The method of serial femtosecond crystallography (SFX) has pushed the frontiers of protein crystallography at X-ray FELs through the use of smaller crystals than typically used with conventional sources and the use of the unique time resolution afforded by X-ray FELs131415. For SFX to contribute novel structural information, routine de novo phasing from X-ray FEL data is necessary. Extending the Se-SAD phasing ‘magic bullet' of structural biology to SFX experiments promises to provide a routine method for de novo phasing at X-rays FELs.

Here we show the successful use of single-wavelength anomalous diffraction to solve the crystal structure of streptavidin bound to a selenobiotin molecule to 1.9 Å. LCLS was operated at energies not previously available, delivering the 12.8 keV X-rays necessary for the work. The Se-B SA co-crystals proved to be a challenging system with which to attempt Se-SAD for the first time using SFX at LCLS. It has a low ratio of selenium per asymmetric unit (one selenium atom per 128 amino acids) and low lattice symmetry (P21), meaning the measureable anomalous difference signal was quite small. The introduction of the sample using the coMESH injector allowed for relatively low sample consumption (<15 mg of protein was used during 18 h of combined data collection time). The coMESH was compatible with the moderately viscous mother liquor composition of 24% PEG 1,500 and 20% glycerol; however, it has increased background, and the associated fluctuations in the background level added to the challenging nature of the data. The measured <ΔF>/<F> was ∼1% at 2 Å resolution. In addition to the weak <ΔF>/<F> for the system, no alpha helices were present in the molecule, making the density modification steps challenging and also rendering solutions using automated pipelines ineffective. These challenges necessitated the use of over 300,000 indexed patterns to achieve the successful phasing of the structure. For these reasons, demonstrating that the data for such a challenging system could be used for successful de novo structure determination indicates a good possibility for general applicability of Se-SAD de novo phasing at LCLS.

>GITGTWYNQLGSTFIVTAGADGALTGTYESAVGNAESRYVLTGRYDSAPATDGSGTALGWTVAWKNNYRNAHSATTWSGQYVGGAEARINTQWLLTSGTTEANAWKSTLVGHDTFTKVKP[4x]> GSHMPSKAKVAIVGSGNISTDLLYKLLRSEWLEPRWMVGIDPESDGLARAAKLGLETTHEGVDWLLAQPDKPDLVF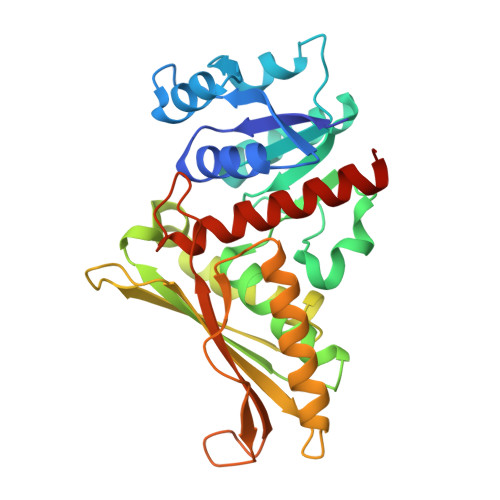EATSAYVHRDAAPKYAEAGIRAIDLTPAAVGPAVIPPANLREHLDAPNVNMITCGGQATIPIVYAVSRIVEVPYAEIVASVASVSAGPGTRANIDEFTKTTARGVQTIGGAARGKAIIILNPADPPMIMRDTIFCAIPTDADREAIAASIHDVVKEVQTYVPGYRLLNEPQFDEPSINSGGQALVTTFVEVEGAGDYLPPYAGNLDIMTAAATKVGEEIAKETLVVGGAR2,4,6-trichlorophenol | C6 H3 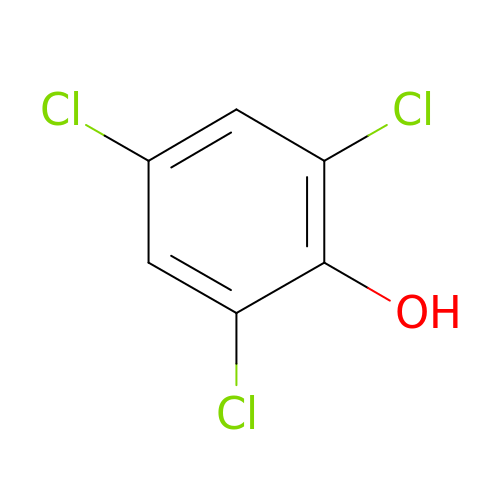Cl3 O | LINPIYWFGCPVIE-UHFFFAOYSA-N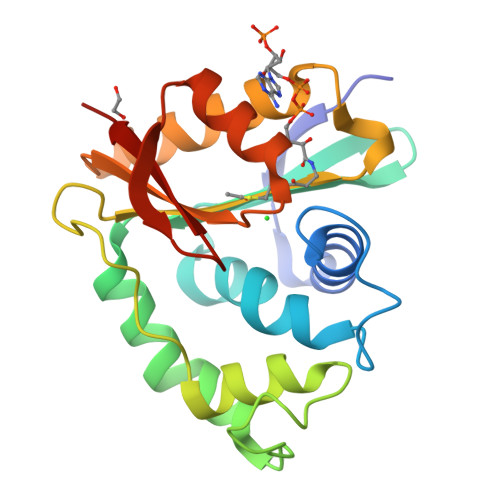> MASEVVIRRATAADHGDLCRVCLLTGDSGRDASSREDDPTLLGMIYAVPYQVGAPDFAFVLEDAEGVCGYLLGAPDTLSFQHFLEKEWLPPLRAGLTDPGPDPAAWQGSDWARDAIHRPPALPPIDLAAYPAHGHIDLLPRAQGRGVGSRAMDHLEAALAAAGAPGMHLQVSPENPRALGFYEHRGFRELCRSEDEVVVGRRLLDE>MRKNIVAGNWKMNLNFEEGQKLTSEIVNMIRDENIKDVSVVLNPPYVHLHPVKKLIGNTAGLFLGAQNCSDKTSGAYT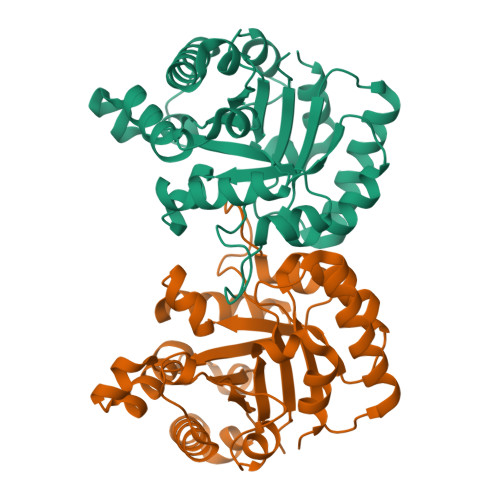GEISASMLASFGSTFVIIGHSERREYFKEDSALLTGKLTQALENGLTPIFCCGESLDIREAGTHEEYVKQQLTESLFGLSATDFAKIVIAYEPIWAIGTGKTASSDQAQEMHAAIRTHLASKYGQAAADEISILYGGSCNPGNAKEIFSKPDVDGGLIGGASLKSRDFLDIIKSF[2x]>SNAMNTTVEKQQIITSNTEQWKMYSKLEGKEYQIHISKPKQPAPDSGYPVIYVLDGNAFFQTFHEAVKIQSVRAEKTGVSPAIIVGVGYPIEGAFSGEERCYDFTPSVISKDAPLKPDGKPWPKTGGAHNFFTFIEEELKPQIEKNFEIDKGKQTLFGHSLGGLFALHILFTNLNAFQNYFISSPSIWWNNKSVLEKEENLIIELNNA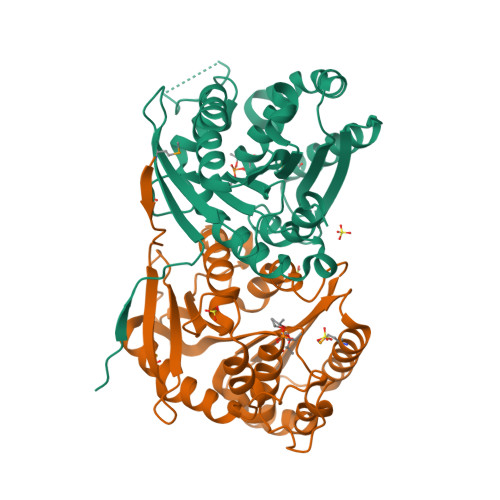KFETGVFLTVGSLEREHMVVGANELSERLLQVNHDKLKFKFYEAEGENHASVVPTSLSKGLRFISYV[2x]Following transfer of IncF-like plasmids, recipients become refractory to a second wave of conjugation with the same plasmid via entry (TraS) and surface (TraT) exclusion mechanisms. SFX, which is mediated by the OMP TraT, is specific for Gram-negative bacteria. TraT is a highly expressed ~24 kDa lipoprotein with a copy number of approximately 29,000–84,000 copies/cell. In this work, we determined the cryo-EM structure of TraT encoded by pKpQIL (TraTpKpQIL) and the F (TraTF) plasmid derivative, pOX38, at 2.47 Å and 2.66 Å resolution respectively. This revealed that lipidated TraT oligomerises into a decameric champagne cork-like structure, composing of a transmembrane α-helical barrel domain and an extracellular ring domain.

To study the structural basis of SFX specificity, the structure of TraTF was also determined. The cryo-EM structure has an overall resolution of 2.66 Å (Fourier shell correlation (FSC) = 0.143 criterion; Fig. 5a, Supplementary Fig. 4 and Supplementary Table 1). Like TraTpKpQIL, TraTF consists of ten identical protomers that form a transmembrane α-helical barrel domain and an extracellular ring-like domain. The TraTF monomer comprises the same secondary structure elements as shown for TraTpKpQIL and exhibits a similar conformation. TraTpKpQIL and TraTF can be superimposed with an rmsd of 0.523 Å over 225 Cα atoms. While TraTpKpQIL and TraTF (85% amino acid identity) exhibit SFX plasmid specificity, their structures are highly conserved. Interestingly, most of the amino acid differences in the TraTF are predominantly smaller side chains such as alanine or glycine residues without changing the charge profile of the β-sandwich domain; no changes are found inside the TraT cavity, suggesting that the β-sandwich domain is likely the site of possible interaction with partner proteins from the donor. The conjugation frequency of pKpQIL into ICC8001-pBAD-traTF and ICC8001-pBAD-empty recipients did not display significant differences, suggesting that TraTF cannot exclude pKpQIL. Although our data together with previous work indicate that MPS and the pilus are not part of the SFX process, the subtle amino acid differences between the TraT sequences provide the high degree of specificity. It is likely that specificity is driven by either the α2 or/and β-hairpin motif as the amino acids display low conservation.

>CGAMSTAIKKRNLEVKTQMSETIWLEPASERTVFLQIKNTSDKDMSGLQGKIADAVKAKGYQVVTSPDKAYYWIQANVLKADKMDLRESQGWLNRGYEGAAVGAALGAGITGYNSNSAGATLGVGLAAGLVGMAADAMVEDVNYTMITDVQIAERTKATVTTDNVAALRQGTSGAKIQTSTETGNQHKYQTRVVSNANKVNLKFEEAKPVLEDQLAKSIANILGS[10x]SOS1 is one of the major guanine nucleotide exchange factors that regulates the ability of KRAS to cycle through its “on” and “off” states. One of the major regulators of this process is the Son of Sevenless (SOS) protein, a guanine nucleotide exchange factor (GEF) that acts as a key activator for KRAS function. The binding between KRAS and SOS proteins helps facilitate the turnover of GDP-loaded KRAS into its GTP-loaded state. Additionally, functional genomic screens have identified that several cancer cell lines addicted to KRAS signaling are particularly sensitive to genetic perturbation of SOS1.15 Functionally, KRAS mutations lead to a reduction in GTPase activity, resulting in a higher population of GTP-bound KRAS and increased RAS-pathway signaling. GTP-bound KRAS also binds to an allosteric site on SOS1, leading to an increase in SOS1 GEF activity, thereby ensuring a high population of active KRAS. Herein, we report the design of a new class of phthalazine-based SOS1 binders that effectively disrupt the SOS1:KRAS protein–protein interaction.

As expected from our modeling efforts, the phthalazine core makes a π-stacking interaction with His905, and the N–H from the C1-benzyl amine substituent creates a crucial hydrogen bond with Asn879. The chiral α-methyl on the benzylic amine fills a small cavity in the pocket and positions the phenyl group for an edge-to-face interaction with Phe890. The ideal C7-substituent should extend from the SOS1 binding pocket into the interface of the KRAS:SOS1 protein–protein interaction between the Arg73 of KRAS and Asn879/Tyr884 of SOS1, thereby disrupting the PPI, while also providing favorable drug-like properties. The C7-piperazine protrudes out of the binding pocket and into the region where the SOS1:KRAS PPI occurs, driving the disruption of the SOS1:KRAS complex. Interestingly, based on atomic distances in the crystal structure, the nitrogen on the 3-position of the phthalazine core is clearly protonated and makes a salt bridge with the carboxylate of Glu902. This is in stark contrast to the previously reported quinazoline-based SOS1 binders that require a methyl group in this position and are unable to utilize this interaction. Finally, the C4-methyl substituent protrudes into the solvent front, which indicated that this vector could be used as an additional opportunity for growth and further tuning of the physicochemical properties of our phthalazine scaffold. Further modeling using the co-crystal structure of compound 15 suggested that a small hydrophilic hole existed in the back pocket of the protein and incorporation of more polar substituents on the phenyl ring may be tolerated. X-ray co-crystal structures of these inhibitors reveal a unique salt bridge between the phthalazine core and Glu902 of SOS1 that has not been reported with previous SOS1 binders.

> GEEQMRLPSADVYRFAEPDSEENIIFEENMQPKAGIPIIKAGTVIKLIERLTYHMYADPNFVRTFLTTYRSFCKPQELLSLIIERFEIPEPEPTEADRIAIENGDQPLSAELKRFRKEYIQPVQLRVLNVCRHWVEHHFYDFERDAYLLQRMEEFIGTVRGKAMKKWVESITKIIQRKKIARDNGPGHNITFQSSPPTVEWHISRPGHIETFDLLTLHPIEIARQLTLLESDLYRAVQPSELVGSVWTKEDKEINSPNLLKMIRHTTNLTLWFEKCIVETENLEERVAVVSRIIEILQVFQELNNFNGVLEVVSAMNSSPVYRLDHTFEQIPSRQKKILEEAHELSEDHYKKYLAKLRSINPPCVPFFGIYLTNILKTEEGNPEVLKRHGKELINFSKRRKVAEITGEIQQYQNQPYCLRVESDIKRFFENLNPMGNSMEKEFTDYLFNKSLEIEPRNPKPLPRFPKKYSYPLKSPGVRPSNPRPGT> CDIHVL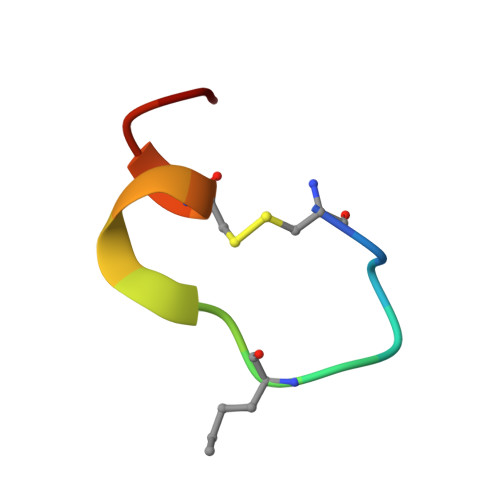WEWECFEKL> PVAKVEPIKIMLKPGKDGPKLRQWPLTKEKIEALKEICEKMEKEGQLEEAPPTNPYNTPTFAIKKKDKNKWRMLIDFRELNKVTQDFTEIQLGIPHPAGLAKKRRITVLDVGDAYFSIPLHEDFRPYTAFTLPSVNNAEPGKRYIYKVLPQGWKGSPAIFQHTMRQVLEPFRKANKDVIIIQYMDDILIASDRTDLEHDRVVLQLKELLNGLGFSTPDEKFQKDPPYHWMGYELWPTKWKLQKIQLPQKEIWTVNDIQKLVGVLNWAAQLYPGIKTKHLCRLISGKMTLTEEVQWTELAEAELEENRIILSQEQEGHYYQEEKELEATVQKDQDNQWTYKIHQEEKILKVGKYAKVKNTHTNGIRLLAQVVQKIGKEALVIWGRIPKFHLPVEREIWEQWWDNYWQVTWIPDWDFVSTPPLVRLAFNLVGDPIPGAETFYTDGSCNRQSKEGKAGYVTDRGKDKVKKLEQTTNQ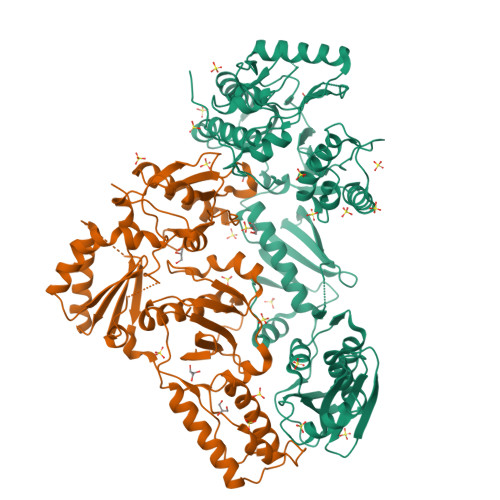QAELEAFAMALTDSGPKVNIIVDSQYVMGIVASQPTESESKIVNQIIEEMIKKEAIYVAWVPAHKGIGGNQEVDHLVSQGI;> EPIKIMLKPGKDGPKLRQWPLTKEKIEALKEICEKMEKEGQLEEAPPTNPYNTPTFAIKKKDKNKWRMLIDFRELNKVTQDFTEIQLGIPHPAGLAKKRRITVLDVGDAYFSIPLHEDFRPYTAFTLPSVNNAEPGKRYIYKVLPQGWKGSPAIFQHTMRQVLEPFRKANKDVIIIQYMDDILIASDRTDLEHDRVVLQLKELLNGLGFSTPDEKFQKDPPYHWMGYELWPTKWKLQKIQLPQKEIWTVNDIQKLVGVLNWAAQLYPGIKTKHLCRLISGKMTLTEEVQWTELAEAELEENRIILSQEQEGHYYQEEKELEATVQKDQDNQWTYKIHQEEKILKVGKYAKVKNTHTNGIRLLAQVVQKIGKEALVIWGRIPKFHLPVEREIWEQWWDNYWQVTWIPDWDFVSTPPLVRLAFNLVGD>ETVPLILLVPKSRREDLEKAQLAERMRSQFFIDYGVRLPEVLLRDGEGLDDNSIVLLINEIRVEQFTVYFDLMRVVNYSDEVVSFGINPTIHQQGSSQYFWVTHEEGEKLREMGYVLRNALDELYHCLAVTLARNVNEYFGIQETKHMLDQLEAKFPDLLKEVLRHAT[2x]

Protein type III secretion systems (T3SSs) are organic nanosyringes that achieve an energy-dependent translocation of bacterial proteins through the two membranes of Gram-negative organisms. InvA is a member of a set of several inner membrane proteins that form this core of the T3SS. Highly conserved across pathogenic bacteria, as well as with a conserved homolog in the flagellar system (FlhA), InvA is critical to the functioning of the T3SS. InvA of S. typhimurium is 685 amino acids in length and the N-terminal 300 amino acids are comprised of seven transmembrane helices.

To begin to address some of these outstanding questions, we determined the crystal structure of a C-terminal fragment of InvA to 1.9 Å resolution. The construct 356–525 produced crystals that diffracted well and allowed the high-resolution structural determination of roughly half of the InvA cytoplasmic domain. The biological significance of this dimer is uncertain, as the protein migrates as a monomeric species on size-exclusion chromatography and the buried surface area of this interaction is less than 500 Å2. The two copies of the protein are very similar, with a root-mean-square deviation in Cα positions of 0.8 Å. Two regions of the protein contribute most to this variation: the C-terminal helix of the truncated construct and an extended region of 30 amino acids spanning residues 370–400. In this latter extended region, covering two helices and a loop, there are overall small translational shifts in the helices in the alignment and in once place, involving residues 390–399, the long loop between H2 and β2 adopts very different conformations, both of which are well ordered in the electron-density maps. Interestingly, the first InvA subdomain (residues 358–417) also has a core with two α-helices and a three-stranded β-­sheet, two strands of which are parallel. The folds are distinct, however, in their topology, with one domain having a βαββα fold (strand–helix–strand–strand–helix) and the other having an αββαβ fold (helix–strand–strand–helix–strand). The second InvA subdomain falls into the former class.(1R,2R,3S,5R,6S)-2,3,5-trihydroxy-6-(hydroxymethyl)cyclohexyl 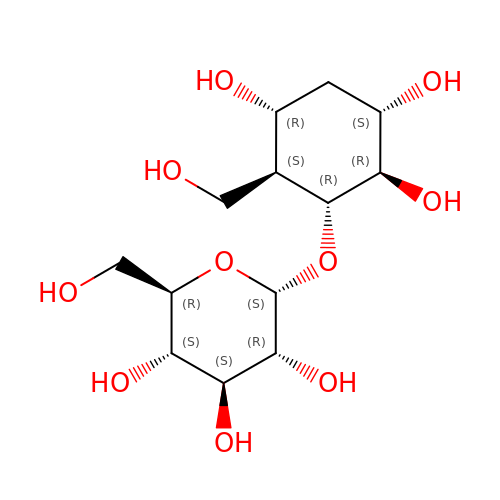alpha-D-glucopyranoside | C13 H24 O10 | POWCVSWKDOOEBI-FELRGSJNSA-N> MAHHHHHHMATGFYSHADCLQHEMGQWHPECPARLQAIEDQLIASRIGELIERESAPLADEAALLRVHTKAHVDYLRARSPQSGYAEID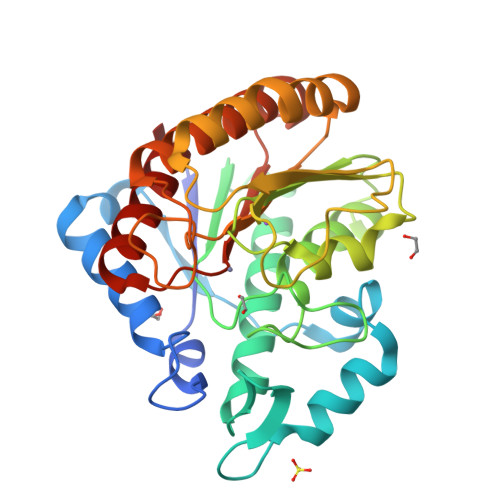PDTSMNPHTWTAALRAAGAAVAATDAVIEGRYDNAFCSVRPPGHHAEPARAMGFCFFNNVAIAARHALEVHKLERVAIIDFDVHHGNGTEAAFSNDARVLMCSIFQHPFYPFTGADNQAPNMCNVPIAARSKGMVVREAIDMIWLPRLDAFKPQMLFVSAGFDAHREDDLGNMALVEDDYAWITQQIRLVADKYAKGRIVSCLEGGYNLSALGRSVVAHVRALADI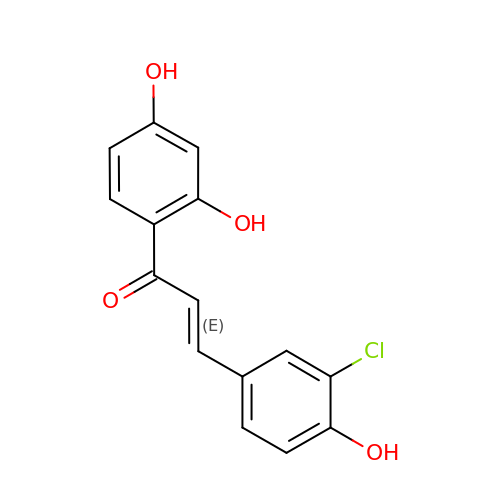(~{E})-1-[2,4-bis(oxidanyl)phenyl]-3-(3-chloranyl-4-oxidanyl-phenyl)prop-2-en-1-one | C15 H11 Cl O4 | ROHDVIDCQSNCQQ-ORCRQEGFSA-N> HGHHSHGKPLTEVEQKAANGVFDD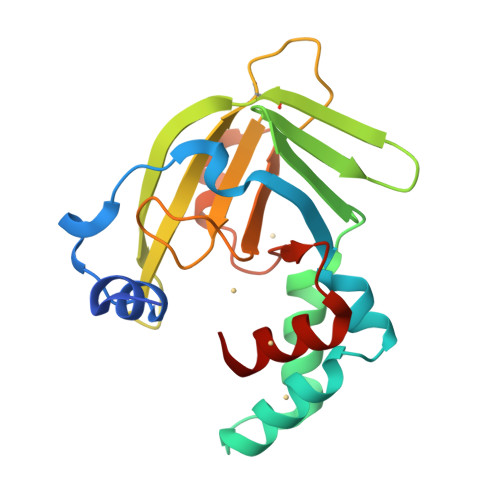ANVQNRTLSDWDGVWQSVYPLLQSGKLDPVFQKKADADKTKTFAEIKDYYHKGYATDIEMIGIEDGIVEFHRNNETTSCKYDYDGYKILTYKSGKKGVRYLFECKDPESKAPKYIQFSDHIIAPRKSSHFHIFMGNDSQQSLLNEMENWPTYYPYQLSSEEVVEEMMSH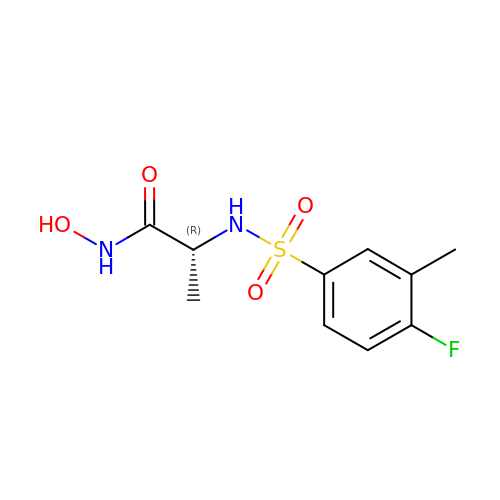N~2~-[(4-fluoro-3-methylphenyl)sulfonyl]-N-hydroxy-D-alaninamide | C10 H13 F N2 O4 S | PGNDHTMCXOFNMS-SSDOTTSWSA-N> GPMGSMNNNEPDTLPDPAIGYIFQNDIVALKQAFSLPDIDYADISQREQLAAAL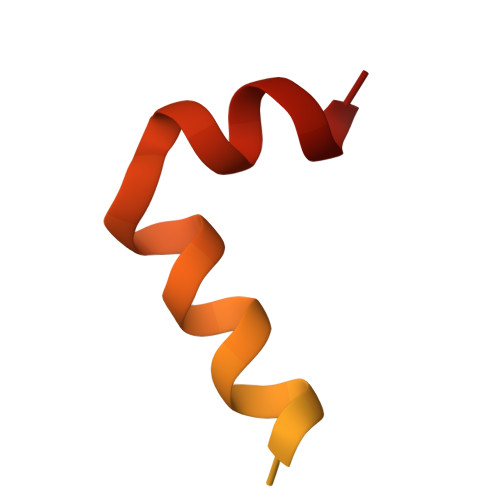KRWPLLAEFAQQK>GPSNLKDFSQPGSGQESNFGVDFVIHYKVPAAERDEAEAGFVQLIRALTTVGLATEVRHGENESLLVFVKVASPDLFAKQVYRARLGDWLHGVRVSAPHNDIAQALQDEPVVEAERLRLIYLMITKPHNEGGAGVTPTNAKWKHVESIFPLHSHSFNKEWIKKWSSKYTLEQTDIDNIRDKFGESVAFYFAFLRSYFRFLVIPSAFGFGAWLLLGQFSYLYALLCGLWSVVFFEYWKKQEVDLAVQWGVRGVSSIQQSRPEFEWEHEAEDPITGEPVKVYPPMKRVKTQLLQIPFALACVVALGALIVTCNSLEVFINEVYSGPGKQYLGFLPTIFLVIGTPTISGVLMGAAEKLNAMENYATVDAHDAALIQKQFVLNFMTSYMALFFTAFVYIPFGHILHPFLNFWRATAQTLTFSEKELPTREFQINPARISNQMFYFTVTAQIVNFATEVVVPYIKQQAFQKAKQLKSGSKVQEDHEEEAEFLQRVREECTLEEYDVSGDYREMVMQFGYVAMFSVAWPLAACCFLVNNWVELRSDALKIAISSRRPIPW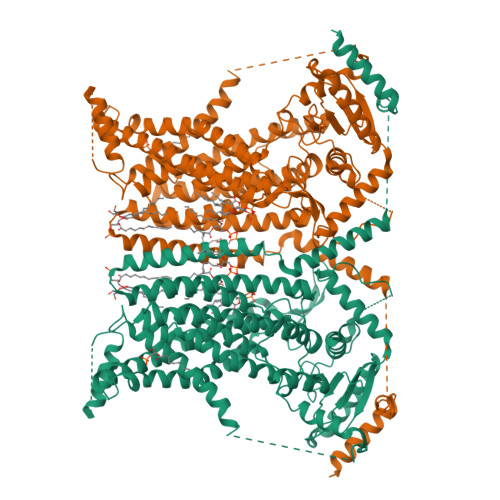RTDSIGPWLTALSFLSWLGSITSSAIVYLCSNSKNGTQGEASPLKAWGLLLSILFAEHFYLVVQLAVRFVLSKLDSPGLQKERKERFQTKKRLLQENLGQDAAEEAAAPGIEHSEKITREALEEEARQASIRGHGTPEEMFWQRQRGMQETIEIGRRMIEQQLAAGKNGKKSAPAVPSEKASA[2x]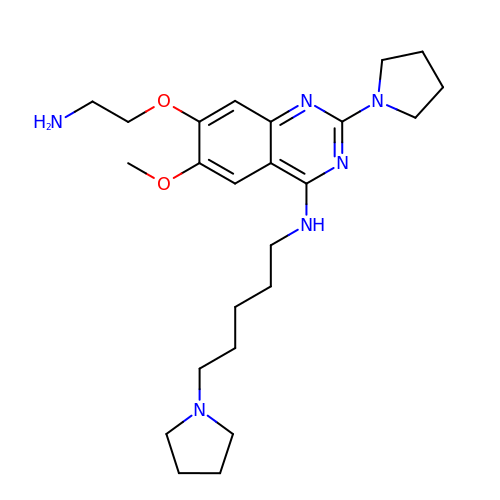7-(2-aminoethoxy)-6-methoxy-2-(pyrrolidin-1-yl)-N-[5-(pyrrolidin-1-yl)pentyl]quinazolin-4-amine | C24 H38 N6 O2 | UEDAXBZCRLISHC-UHFFFAOYSA-N The anti-apoptotic (pro-survival) proteins of the BCL-2 family include BCL-2, BCL-XL, MCL-1, BCL-w and BFL-1/A1. These proteins bind to and sequester the apoptosis effectors, as well as the apoptosis sensitizers, BIM, BID, PUMA, NOXA, BAD, BMF, HRK and BIK5,6. An elongated hydrophobic groove is thus formed along the surface of BCL-2 and BCL-XL proteins, spanning approximately 20 Å to serve as the binding site for the amphipathic α-helical BH3 domains of their pro-apoptotic partners. Herein we present cyclic peptides (CPs) with nanomolar-level binding affinities to BCL-2 or BCL-XL, and further reveal the structural and functional mechanisms of how these CPs target two proteins in a fashion that is remarkably different from traditional small-molecule inhibitors.

As the long-term clinical application of venetoclax has caused an occurrence of drug-resistant BCL-2 mutations (such as G101V and D103Y), it is critical to seek for inhibitors potentially overcoming them and figure out the mechanism of action. To examine this hypothesis, we obtained the crystals of BCL-2 G101V mutant in complex with cp1 that diffracted to a high resolution (1.85 Å) in space group P21. The overall structure of BCL-2 G101V is similar to WT, except for the N-terminus of α4 helix, which is relatively far away from the cp1 binding site, and is likely not directly involved in the binding of cp1 to G101V mutant. The electron density of cp1 in BCL-2 G101V complex was also well defined, showing a highly similar conformation for cp1 as in the WT structure. However, the minimum distance between E152 and cp1 is about 7.7 Å, much further than those between E152 and venetoclax or S55746 in their complexes with BCL-2 G101V mutant, 3.3 Å and 3.9 Å, respectively. This distance difference suggests that the knock-on effect of G101V mutation on the adjacent E152, which accounts for its drug resistance to venetoclax or S55746 as previously illustrated, may not drastically impact the binding of cp1 to the BCL-2 G101V mutant. To confirm this, an SPR assay was conducted and the results showed that the affinity of cp1 to BCL-2 G101V mutant was 1.00 ± 0.13 μM (close to the 0.65 ± 0.14 μM for BCL-2 WT), indicating no drastic influence on cp1 binding. Interestingly, in the BCL-2 G101V-cp1 complex we found the conformational change of E152 residue may further lead to a 90° rotamer change of neighboring F112, as compared with its counterpart in the WT-cp1 complex. Probably as an accommodated move, the nearby F104 residue on α2 also shows a 90° rotamer change, which is not observed in the complex structures of BCL-2 WT-cp1, G101V-venetoclax and G101V-S55746. These results indicate that the BCL-2 mutation G101V may not only influence the conformation of E152 as previously reported, but also cause conformational changes of F112 and F104.

> MAHAGRTGYDNREIVMKYIHYKLSQRGYEWDAGDDVEENRTEAPEGTESEVVHLTLRQAVDDFSRRYRRDFAEMSSQLHLTPFTARGRFATVVEELFRDGVNWGRIVAFFEFGGVMCVESVNREMSPLVDNIALWMTEYLNRHLHTWIQDNGGWDAFVELYGPSMR;> CPARYGWDYECX>[2x]MTQDVTSGYSNLDLDLRDNGVCVVTLNRPDKRNALDVATIEELVTFFSTAHRKGVRAVVLTGAGDHFCAGLDLVEHWKADRSADDFMHVCLRWHEAFNKMEYGGVPIIAALRGAVVGGGLALASAAHLRVMDQSTYFALPEGQRGIFTGGGATIRVSDMIGKYRMIDMILTGRVYQGQEAADLGLAQYITEGSSFDKAMELADKIASNLPLTNFAICSAISHMQNMSGLDAAYAEAFVGGIVNTQPAARERLEAFANKTAARVRPNSLEHHHHHH

The enzyme DmdD catalyzes the last step of the MeSH pathway, the hydration and hydrolysis of MTA-CoA. DmdD belongs to the crotonase superfamily of enzymes, homologous to the equivalent enzyme in the fatty acid β-oxidation pathway. The structure of the DmdD monomer contains two domains. Consistent with the gel-filtration data, DmdD is a hexamer in the crystal, which is also similar to the architecture of canonical crotonases.

The crystal structure of wild-type R. pomeroyi DmdD free enzyme has been determined at 1.5 Å resolution by the molecular replacement method. To determine the structure of DmdD in complex with its substrate, we created the catalytically inactive E121A mutant (see below). Crystals of this mutant were soaked with MTA-CoA or MMPA-CoA, and the structures of the two complexes were determined at 1.8 Å resolution. Good-quality electron density was observed for both MTA-CoA molecules in the crystal. However, there are differences in their binding modes in the two molecules of DmdD. In the first molecule (molecule 1 in Fig. 3A), the entire MTA-CoA molecule is inserted into a deep active site pocket on the surface of DmdD (to be referred to as binding mode A), formed primarily by residues in one monomer (α2, α3, α10, β5-α2 loop, and β9-α5 loop) but also with contributions from the CTD (α10, α11 and the C-terminal loop) of a neighboring monomer of the trimer. The phosphate groups of CoA are recognized by ionic interactions with Lys31, Arg32, and His66. Moreover, the C-terminal loop of the neighboring monomer provides three additional side chains, Lys258′, Arg262′ and Arg264′, for ionic interactions with the phosphate groups. For example, the long loop at the C-terminus of DmdD is observed only in one of the two monomers in the MTA-CoA complex, where it is involved in binding the substrate. In addition, the C-terminal loop and part of helix α11′ of the neighboring monomer are not ordered in the active site for binding mode B, which leaves the phosphate groups of CoA exposed to the solvent. The carbonyl oxygen of MTA is hydrogen-bonded to the main-chain amides of Leu71 and Gly118, the oxyanion hole of this enzyme.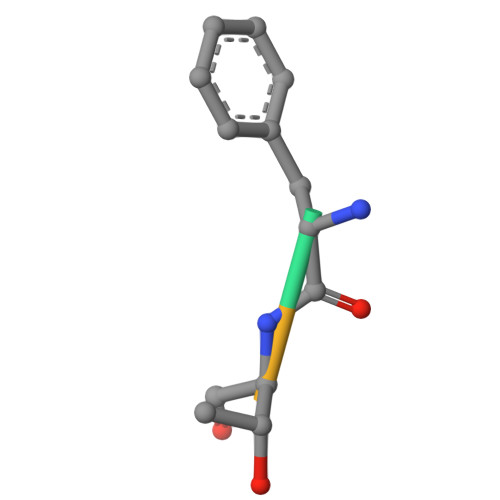> FTAG>[2x]QKHLNEKQQENQDLLVKCISQNLGYNGDKPVAACVIYKCLLHWRSF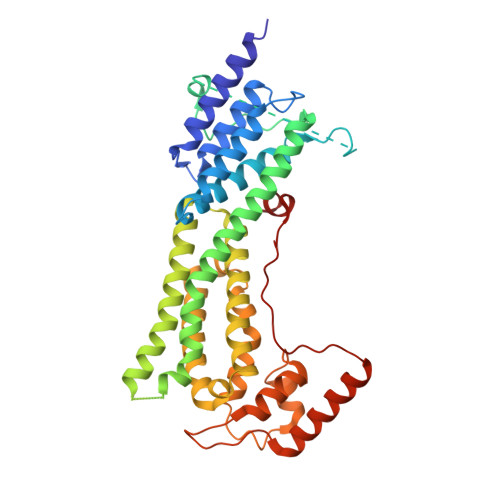EVERTSVFDRIIQTIATAIEVPDNNEVLAYWLSNSATLLLLLQRTLKATGAASLTPQRRRTTSASLFGRMSQGLRGSPQSAGLSFLNRQGLTKLDDLRQVEAKYPALLFKQQLTAFLEKIYGMIRDNLKKEISPLLGLCIQAPRTSRASLVKGRAQANAVAQQALIAHWQSIRKSLNSYLNLMKANNAPPFLVRKVFTQIFSFINVQLFNSLLLRRECCSFSNGEYVKAGLAELEQWCIEATDEYAGSAWDELRHIRQAVGFLVIHQKPKKTLDEITRELCPVLSIQQLYRISTMYWDDKYGTHSVSSDVIANMRVMMTEDSNNAVSSSFLLDDDSSIPFTVEDISKSM> MKDLVDTTEMYLRTIYELEEEGVTPLRARIAERLEQSGPTVSQTVARMERDGLVVVASDRSLQMTPTGRTLATAVMRKHRLAERLLTDIIGLDINKVHDEADRWEHVMSDEVERRLVKVLKDVSRSPFGNPIPGLDELGVGNSDAAAPGTRVIDAATSMPRKVRIVQINEIFQVETDQFTQLLDADIRVGSEV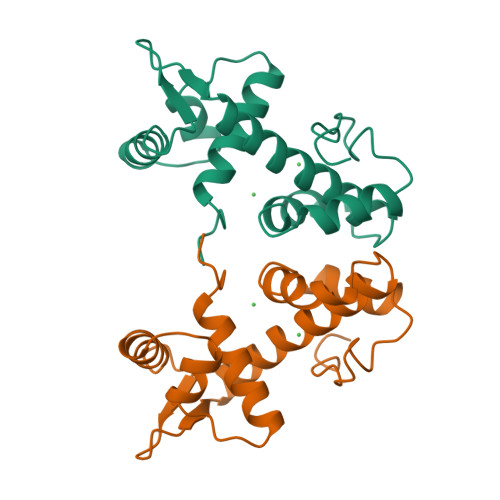EIVDRDGHITLSHNGKDVELLDDLAHTIRIEEL N'-(5-chloro-1,3-benzodioxol-4-yl)-N-(3-methylsulfonylphenyl)pyrimidine-2,4-diamine | C18 H15 Cl 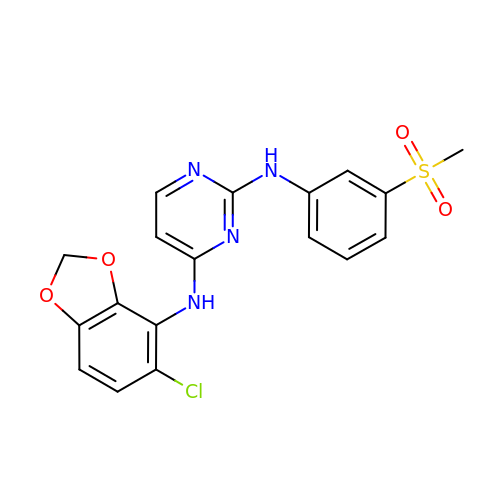N4 O4 S | QTFCKBFCXDAZIU-UHFFFAOYSA-N> SRGASNSSNNNNNNNKVYKRYNSKAKEISRHCVFCENNNEPEAVINSHSVRDNFNRVLCPKLRTYV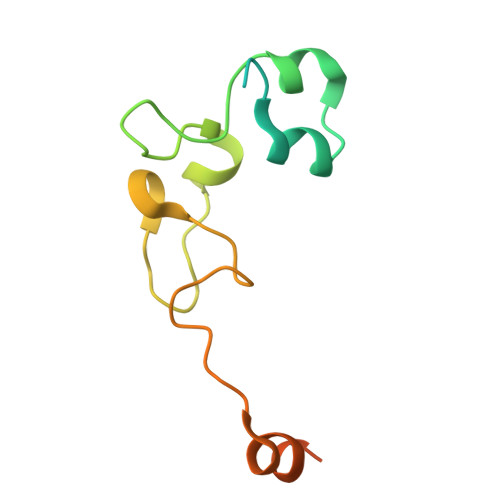CPICGASGDSAHTIKYCPKKPIITMEDAIKAESFRLAKSSYYKQQMKV1-(cyclopentylmethyl)-1-[3-methoxy-4-(2-morpholin-4-ylethoxy)phenyl]-3-[3-(5-methylimidazol-1-yl)propyl]urea | C27 H41 N5 O4 | 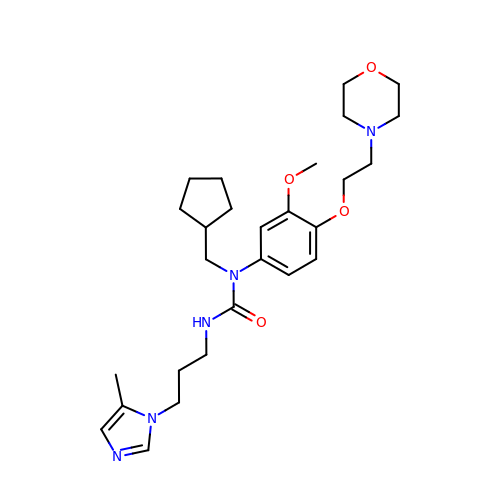FVTOUNXWAFKVHI-UHFFFAOYSA-N> MQDKIPTIAELRELSLRLLTKIPYLKMLVLFGSRATGNINANSD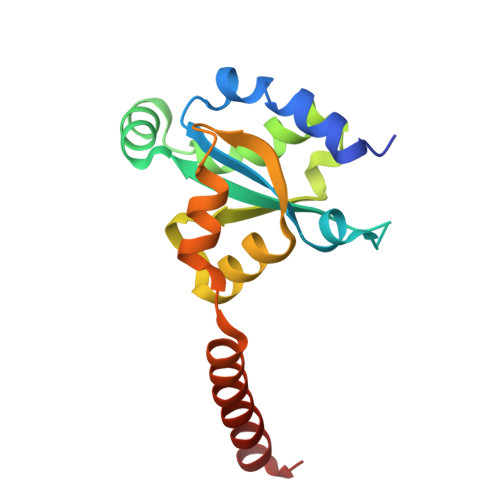WDFAVLYDEEKYNLYIQNNPLAAFVIPGILGEIFKINSDKIDIVELNHCSKLIAHFVARDGKVLYEEPGDEFDKFQQRVLLSNTEIKKIEKTKLENIENFLQRWGV PTase is the key enzyme of the mannose 6-phosphate (M6P) targeting system that is responsible for tagging lysosomal hydrolases with the M6P moiety for their delivery to the lysosome. First, GlcNAc-1-phosphotransferase (PTase) transfers GlcNAc-1-phosphate (GlcNAc-1-P) from UDP-GlcNAc to mannose residues on the high mannose glycans of the hydrolases, following which the GlcNAc moiety is removed by uncovering enzyme to generate the M6P monoester. PTase is an α2β2γ2 heterohexamer encoded by two genes, GNPTAB and GNPTG. The α and β subunits are transcribed and translated from the GNPTAB gene as a precursor molecule that is cleaved by site-1 protease (S1P) at Lys-928 to generate the individual subunits, a critical step for the activation of the molecule.

To determine if this region is necessary, we resolved the cryo-EM structure of hPTase in the presence of the nucleotide donor sugar UDP-GlcNAc at an average resolution of 2.9 Å. The overall architecture shows no major change in the presence, or absence of UDP-GlcNAc, and resembles that of S1S3 and the engineered zPTase. This high-quality EM 3D map permits the entire UDP-GlcNAc molecule to be clearly observable, and as expected, UDP-GlcNAc is in the conserved UDP-sugar binding pocket and binds in a manner highly similar to that in zPTase, with the exception that the two Mg2+ ions are replaced by two Mn2+ ions here. The GlcNAc moiety H-bonds with Glu-389 via the neighboring O3 and O4 hydroxyls. The α-phosphate of the UDP-GlcNAc forms a salt bridge with Arg-322 and Arg-986, and the α- and β-phosphates each contribute an oxygen atom to coordinate with Mn2+ (Mn1), as does Asp-408 (the last residue in the NDD motif) and Asn-1151. Also visible in our structure are the hydrogen bonds between the ribose O2′ and O3′ hydroxyl groups of the UDP-GlcNAc and Thr-80 and Asn-406, respectively. Strikingly, the binding of UDP-GlcNAc extends the ordered structure of the N-termini of CR2 an additional seven residues, from Phe-323 to Glu-316. This converts the deep and large pocket to a flat and shallow one. Thus, the UDP-GlcNAc bound form of the enzyme locks hPTase in an active state, and the phosphoryl transfer can occur once an acceptor glycan chain is inserted into the pocket.

>[2x]DEDQVDPRLIDGKWSRDQYHVLFDSYRDNIAGKSFQNRLCLPMPIDVVYTWVNGTDLELLKELQQVREQMEEEQKAMREILGKNTTEPTKKSEKQLECLLTHCIKVPMLVLDPALPANITLKDLPSLYPSFHSASDIFNVAKPKNPSTNVSVVVFDSTKDVEDAHSGLLKGNSRQTVWRGYLTTDKEVPGLVLMQDLAFLSGFPPTFKETNQLKTKLPENLSSKVKLLQLYSEASVALLKLNNPKDFQELNKQTKKNMTIDGKELTISPAYLLWDLSAISQSKQDEDISASRFEDNEELRYSLRSIERHAPWVRNIFIVTNGQIPSWLNLDNPRVTIVTHQDVFRNLSHLPTFSSPAIESHIHRIEGLSQKFIYLNDDVMFGKDVWPDDFYSHSKGQKVYLTWPVPNCAEGCPGSWIKDGYCDKACNNSACDWDGGDCSGNSGGSRYIAGGGGTGSIGVGQPWQFGGGINSVSYCNQGCANSWLADKFCDQACNVLSCGFDAGDCGQDHFHELYKVILLPNQTHYIIPKGECLPYFSFAEVAKRGVEGAYSDNPIIRHASIANKWKTIHLIMHSGMNATTIHFNLTFQNTNDEEFKMQITVEVDTREGPKLNSTAQKGYENLVSPITLLPEAEILFEDIPKEKRFPKFKRHDVNSTRRAQEEVKIPLVNISLLPKDAQLSLNTLDLQLEHGDITLKGYNLSKSALLRSFLMNSQHAKIKNQAIITDETNDSLVAPQEKQVHKSILPNSLGVSERLQRLTFPAVSVKVNGHDQGQNPPLDLETTARFRVETHTQKTIGGNVTKEKPPSLIVPLESQMTKEKKITGKEKENSRMEENAENHIGVTEVLLGRKLQHYTDSYLGFLPWEKKKYFQDLLDEEESLKTQLAYFTDSKNRARYKRDTFADSLRYVNKILNSKFGFTSRKVPAHMPHMIDRIVMQELQDMFPEEFDKTSFHKVRHSEDMQFAFSYFYYLMSAVQPLNISQVFDEVDTDQSGVLSDREIRTLATRIHELPLSLQDLTGLEHMLINCSKMLPADITQLNNIPPTQESYYDPNLPPVTKSLVTNCKPVTDKIHKAYKDKNKYRFEIMGEEEIAFKMIRTNVSHVVGQLDDIRKNPRKFVCLNDNIDHNHKDAQTVKAVLRDFYESMFPIPSQFELPREYRNRFLHMHELQEWRAYRDKLK> SNAMAKQTIIVMSDSHGDSLIVEEVRDRYVGKVDAVFHNGDSELRPDSPLWEGIRVVKGNMDFYAGYPERLVTELGSTKIIQTHGHLFDINFNFQKLDYWAQEEEAAICLYGHLHVPSAWLEGKILFLNP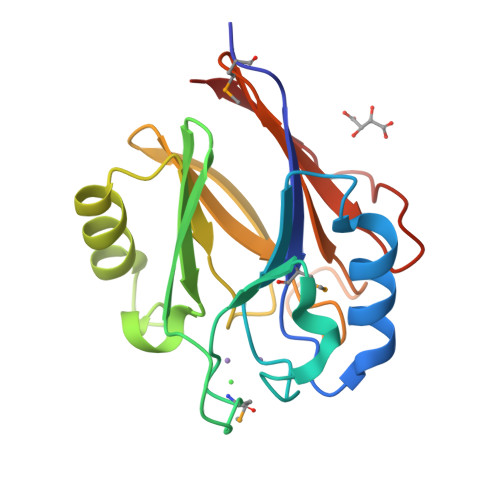GSISQPRGTIRECLYARVEIDDSYFKVDFLTRDHEVYPGLSKEFSR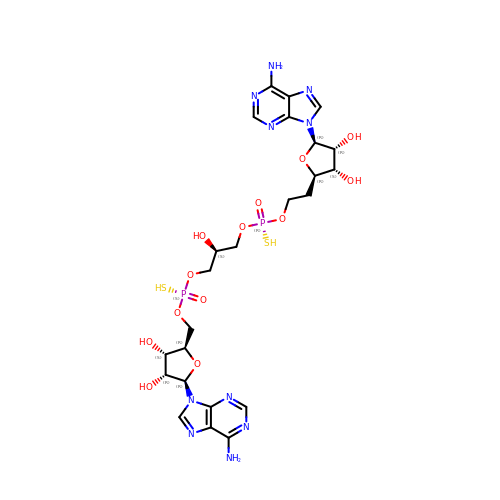(2R,3R,4S,5R)-2-(6-aminopurin-9-yl)-5-[2-[[(2S)-3-[[(2R,3S,4R,5R)-5-(6-aminopurin-9-yl)-3,4-bis(oxidanyl)oxolan-2-yl]methoxy-sulfanyl-phosphoryl]oxy-2-oxidanyl-propoxy]-sulfanyl-phosphoryl]oxyethyl]oxolane-3,4-diol | C24 H34 N10 O13 P2 S2 | OABPMBSLNAAXBR-CZUYOEIMSA-N>[2x]MRVLVVEDN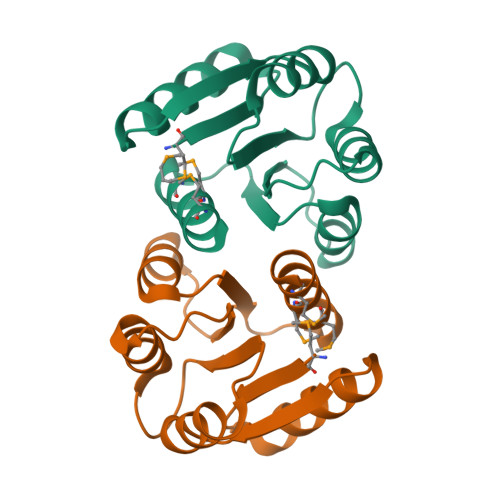ALLRHHLKVQIQDAGHQVDDAEDAKEADYYLNEHIPDIAIVDLGLPDEDGLSLIRRWRSNDVSLPILVLTARESWQDKVEVLSAGADDYVTKPFHIEEVMARMQALMRRNSQ1-[(1R)-1-(3-methoxyphenyl)ethyl]-3-(4-pyridin-4-yl-1,3-thiazol-2-yl)urea 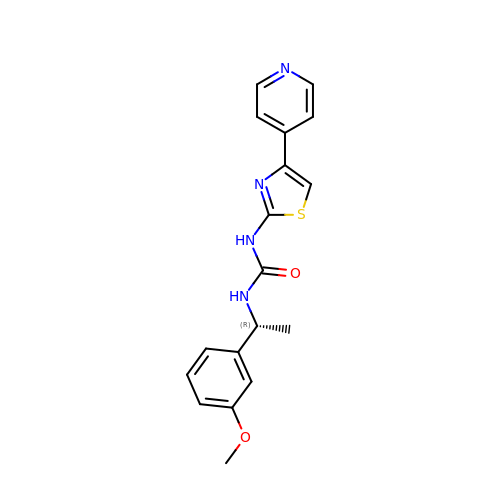| C18 H18 N4 O2 S | PZUHTMLHMMXBQW-GFCCVEGCSA-N> MKKFRKHKRISNCISILLILYLTLGGLLPNNIYAQDLQSYSEKVCNTTYKAPIERPEDFLKDKEKAKEWERKEAERIEQKLERSEKEALESYKKDSVEISKYSQTRNYFYDYQIEANSREKEYKELRNAISKNKIDKPMYVYYFESPEKFAFNKVIRTENQNEISLEKFNEFKETIQNKLFKQDGFKDISLYEPGKGDEKPTPLLMHLKLPRNTGMLPYTNTNNVSTLIEQGYSIKIDKIVRIVIDGKHYIKAEASVVSSLDFKDDVSKGDSWGKANYNDWSNKLTPNELADVNDYMRGGYTAINNYLISNGPVNNPNPELDSKITNIENALKREPIPT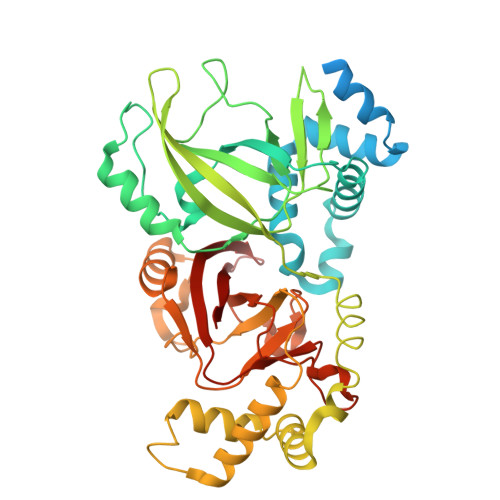NLTVYRRSGPQEFGLTLTSPEYDFNKLENIDAFKSKWEGQALSYPNFISTSIGSVNMSAFAKRKIVLRITIPKGSPGAYLSAIPGYAGEYEVLLNHGSKFKINKIDSYKDGTITKLIVDATLIP>[2x]MANGANRVDLDGKPIQPLTICMIGAGGFIGSHLCEKLLTETPHKVLALDVYNDKIKHLLEPDTVEWSGRIQFHRINIKHDSRLEGLVKMADLIINLAAICTPADYNTRPLDTIYSNFIDALPVVKYCSENNKRLIHFSTCEVYGKTIGSFLPKDHPLRDDPAFYVLKEDISPCIFGSIEKQRWSYACAKQLIERLVYAEGAENGLEFTIVRPFNWIGPRMDFIPGIDGPSEGVPRVLACFSNNLLRRE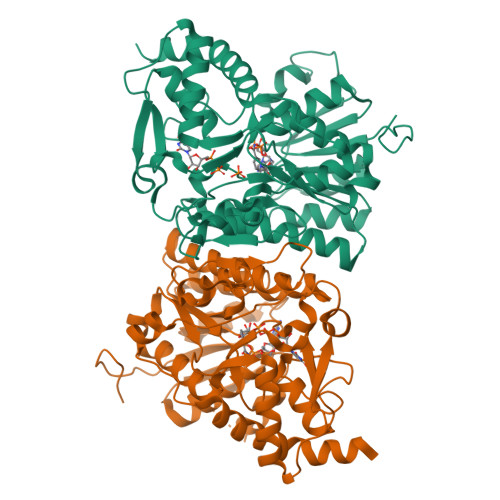PLKLVDGGESQRTFVYINDAIEAVLLMIENPERANGHIFNVGNPNNEVTVRQLAEMMTEVYAKVSGEGAIESPTVDVSSKEFYGEGYDDSDKRIPDMTIINRQLGWNPKTSLWDLLESTLTYQHRTYAEAVKKATSKPVAS>MEPEINCSELCDSFPGQELDRRPLHDLCKTTITSSHHSSKTISSLSPVLLGIVWTFLSCGLLLILFFLAFTIHCRKNRIVKMSSP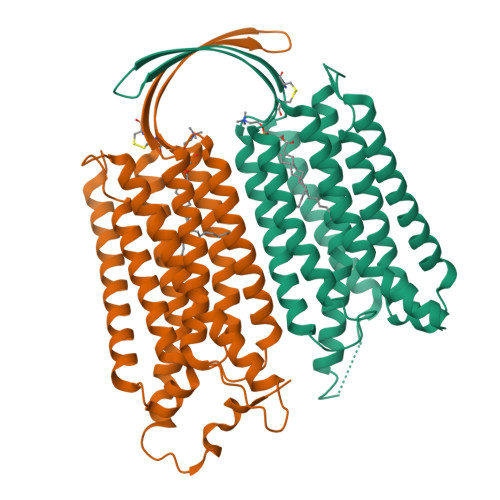NLNIVTLLGSCLTYSSAYLFGIQDVLVGSSMETLIQTRLSMLCIGTSLVFGPILGKSWRLYKVFTQRVPDKRVIIKDLQLLGLVAALLMADVILLMTWVLTDPIQCLQILSVSMTVTGKDVSCTSTSTHFCASRYSDVWIALIWGCKGLLLLYGAYLAGLTGHVSSPPVNQSLTIMVGVNLLVLAAGLLFVVTRYLHSWPNLVFGLTSGGIFVCTTTINCFIFIPQLKQWKAFEEENQTIRRMAKYFSTPNKSFHTQYGEEENCHPRGEKSSMERLLTEKNAVIESLQEQVNNAKEKIVRLMSAECTYDLPEGAAPPASSPNKDVQAVASVHTLAAAQGPSGHLSDFQNDPGMAARDSQCTSGPSSYAQSLEGPGKDSSFSPGKEEKISDSKDFSDHLDSGCSQKPWTEQSLGPERGDQVPMNPSQSLLPERGGSDPQRQRHLENSEEPPERRSRVSSVIREKLQEVLQDLGSGSGSGRGRGGSENLYFQGGSGSGGDYKDDDDKDYKDDDDK[2x]> GAMGSNLLQELTIAKSFGRHQIFLDEARINENPVNRLSRLINTQFWNSLTRRVDLNNVGEIAKDTKIDTPGAKNPRIYVPYDCPEQYEFYVQASQMHPSLKLEVEYLPKKITAEYVKSVNDTPGLLALAMEEHFNPSTGEKTLIGYPYAVPGGRFNELYGWDSYMMALGLLEANKTDVARGMVEHFIFEINHYGKILNANRSYYLCRSQPPFLTEMALVVFKKLGGRSNPDAVDLLKRAFQASIKEYKTVWTASPRLDPETGLSRYHPNGLGIPPETESDHFDTVLLPYASKHGVTLDEFKQLYNDGKIKEPKLDEFFLHDRGVRESGHDTTYRFEGVCAYLATIDLNSLLYKYEIDIADFIKEFCDDKYEDPLDHSITTSAMWKEMAKIRQEKITKYMWDDESGFFFDYNTKIKHRTSYESATTFWALWAGLATKEQAQKMVEKALPKLEMLGGLAACTERSRGPISISRPIRQWDYPFGWAP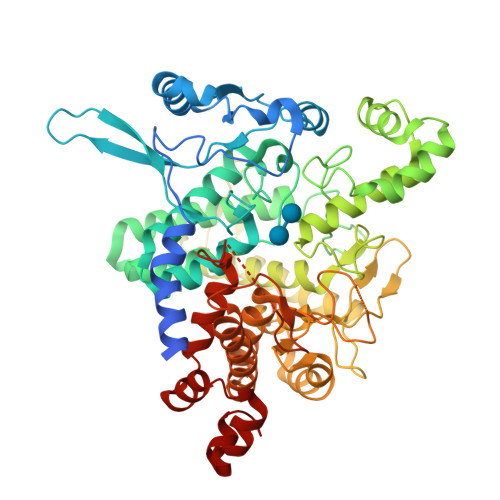HQILAWEGLRSYGYLTVTNRLAYRWLFMMTKAFVDYNGIVVEKYDVTRGTDPHRVEAEYGNQGADFKGAATEGFGWVNASYILGLKYMNSHARRALGACIPPISFFSSLRPQERNLYGL>[3x]MGRPRKDSRLMPVSLSVQSPAALTAEKEAMCLSAPALALKLPIPSPQRAFTLQVSSDPSMYIEVENEVTVVGGVKLSRLKCNREGKEWETVLTSRILTAAGSCDVVCVACEKRMLSVFSTCGRRLLSPILLPSPISTLHCTGSYVMALTAAATLSVWDVHRQVVVVKEESLHSILAGSDMTVSQILLTQHGIPVMNLSDGKAYCFNPSLSTWNLVSDKQDSLAQCADFRSSLPSQDAMLCSGPLAIIQGRTSNSGRQAARLFSVPHVVQQETTLAYLENQVAAALTLQSSHEYRHWLLVYARYLVNEGFEYRLREICKDLLGPVHYSTGSQWESTVVGLRKRELLKELLPVIGQNLRFQRLFTECQEQLDILRDKLEGSS

The presence of the Histone regulator A (HIRA) with the histone variant H3.3 in a soluble complex has implicated this histone chaperone in the specific deposition of this variant. HIRA is in a complex that contains at least two other subunits, Calcineurin-binding protein 1 (CABIN1) and Ubinuclein 1 (UBN1). Furthermore, HIRA serves as a scaffold protein to bring together the other subunits as well as ASF1a. It binds UBN1/2, CABIN1, and ASF1a through its N-terminal WD40 repeat, C-terminal C, and central B domains, respectively.

To determine the molecular basis for HIRA homooligomerization, we determined the crystal structure of the C-terminal half of HIRA (aa 644–1017) at 2.4 Å resolution. The asymmetric unit of the crystal contained a homotrimer of HIRA(644–1017). The observed average value for inter-subunit buried surface area of the homotrimer is ∼1440 Å2,consistent with its high stability. We confirmed the existence of three distinct domains as previously predicted and refined the domain boundaries, β-strand (residues 691–859), loop (residues 860–907), and α-helical (residues 908–1017). N-terminal residues 644–674 were not visible in the crystal structure, suggesting that this region of HIRA(644–1017) is highly flexible. The trimer is arranged in a ring of two layers, composed of β-strands and α-helices, respectively. The β-strand domain is composed of two β-sandwich motifs, β1 (residues 682–774) and β2 (residues 775–860) motifs. Trp799 and/or Asp800, which were identified as critical residues for homotrimer formation, are located in the β2 motif. While Asp800 does not interact with an adjacent subunit, Trp799 is located at the interface of the two subunits and forms a hydrophobic patch with Ile771 and Val806. This hydrophobic patch interacts with Leu851 and Thr853 of an adjacent subunit.>MAHHHHHHMNLRAAGPGWLFCPADRPERFAKAAAAADVVILDLEDGVAEAQKPAARNALRDTPLDPERTVVRINAGGTADQARDLEALAGTAYTTVMLPKAESAAQVIELAPRDVIALVETARGAVCAAEIAAADPTVGMMWGAEDLIATLGGSSSRRADGAYRDVARHVRSTILLAASAFGRLALDAVHLDILDVEGLQEEARDAAAVGFDVTVCIHPSQIPVVRKAYRPSHEKLAWARRVLAASRSERGAFAFEGQMVDSPVLTHAETMLRRAGEATSE[3x]

Mtb protein Rv2498c is currently annotated as the β-subunit (CitE) of the heterotrimeric prokaryotic citrate lyase complex involved in TCA cycle cataplerosis. Combining phylogenetic analysis, in vitro enzymatic assays, in vivo Mtb experiments, and X-ray crystallography, we identified Mtb Rv2498c as an essential stereospecific bifunctional β-hydroxyacyl-CoA lyase (β-HAC lyase) that carries out the last step of itaconate dissimilation pathway and confers resistance to itaconate. A systematic evaluation of substrate specificity revealed (R)-HMG-CoA ∼ (S)-citramalyl-CoA >>> (S)-malyl-CoA ∼ β-methylmalyl-CoA as substrates for Rv2498c. To investigate the molecular basis of Rv2498c substrate stereospecificity for the carbon–carbon bond, we determined the structures of Rv2498c in a variety of liganded states by X-ray crystallography.

In contrast to the previously reported structures, the C terminus (50 residues) is well ordered in our structures, forming an α-helix/β-hairpin/α-helix motif that packs against the surface of the neighboring protomer, capping its active site. Of note, the structure with (S)-citramalyl-CoA bound was obtained from crystals that were soaked with pyruvate and Ac-CoA, therefore indicating that the conformation of Rv2498c in the crystals is catalytically active. The CoA moiety binds in a deep cleft at the base of which resides the active site Mg2+ ion. The Mg2+ ion is coordinated by the 3-hydroxyl group and by an unidentate interaction with the terminal carboxylate of the ligand, as well as by Glu112, Asp138, and 2 water molecules. The carboxylate of the substrate is further positioned by polar interactions with the backbone NH atoms of Ala136, Glu137, and Asp138, while the 3-hydroxyl group lies close to Arg64. The 3-methyl group of the ligand contacts a hydrophobic surface formed by Gly135 and the side-chain atoms of Met133 and Val181. Because the citramalyl group observed in the active site was in the S configuration, which corresponds to the R configuration at the 3-position of HMG-CoA, we modeled the mode of binding of (R)-HMG-CoA to further understand the molecular basis for the (S)-HMG-CoA lyase associated with mammalian l-leucine catabolism. In this case, the additional methylene unit (C4) found in HMG-CoA is readily accommodated in the active site and can support a less distorted octahedral coordination of the Mg2+ ion (the bite angle of the citramalyl group is ∼70°; the modeled HMG moiety bite angle is ∼85°). Our crystal structures for full-length Rv2498c shed light into the molecular basis of substrate specificity and stereoselectivity for (S)-citramalyl-CoA and revealed how the C-terminal domain interacts directly with the neighboring CoA substrate, therefore playing an important role in substrate binding selectivity.> DVDTYLSNLQ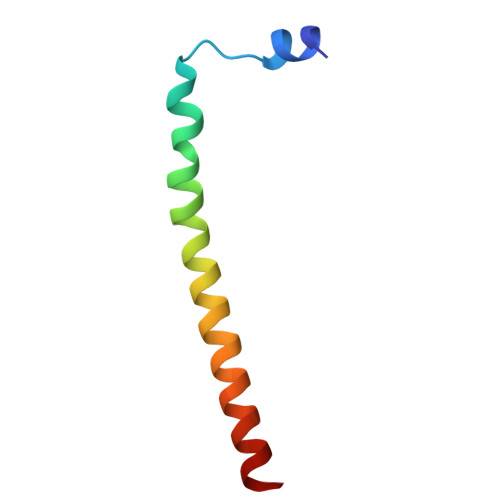TKTTLSMIADGLERSARDFDAFLEENVTLEWEAQRKRIYQHFG> GSAMADIGAEIKQGIREVILCKDQDGKIGLRLKSVDNGIFVQLVQANSPASLVGLRFGDQVLQINGENCAGWSSDKAHKVLKQAFGEKI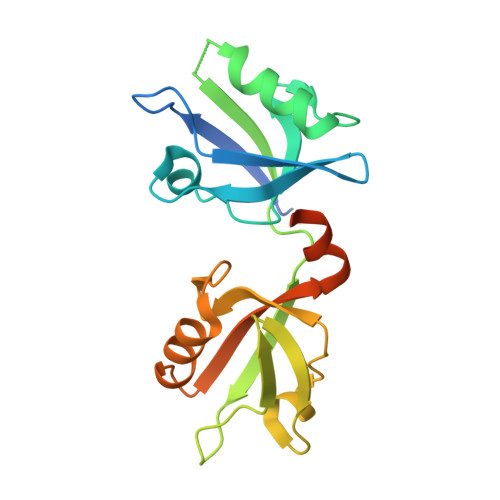TMTIRDRPFERTVTMHKDSSGHVGFIFKSGKITSIVKDSSAARNGLLTDHHICEINGQNVIGLKDAQIADILSTAGTVVTITIMPAFIFEHIIKRMAPSIMKSLMDHTIPEV> GTGGTGGTGGTGT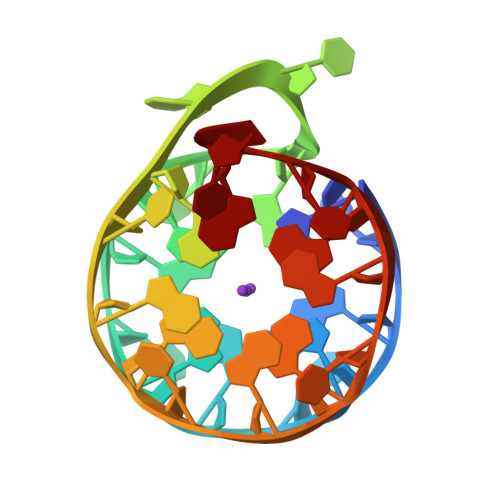TGTGGTGGTGGTGT>ATPHINAEMGDFADVVLMPGDPLRAKYIAETFLEDAREVNNVRGMLGFTGTYKGRKISVMGHGMGIPSCSIYTKELITDFGVKKIIRVGSCGAVLPHVKLRDVVIGMGACTDSKVNRIRFKDHDFAAIADFDMVRNAVD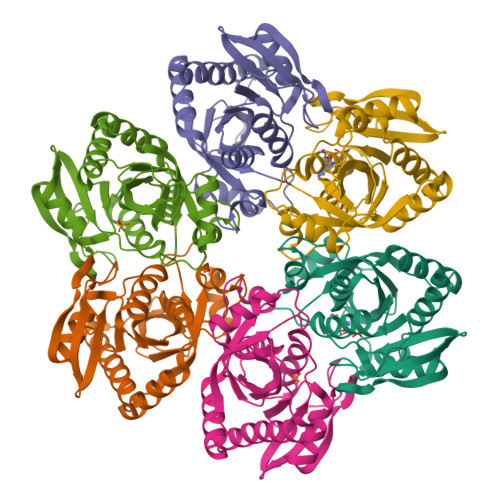AAKALGIDARVGNLFSADLFYSPDGEMFDVMEKYGILGVEMEAAGIYGVAAEFGAKALTICTVSDHIRTHEQTTAAERQTTFNDMIKIALESVLLGDK[6x]> MASWSHPQFEKGAMKHREIRYTDGHTQFVGELHWDEQQGGKCPGVVVFPEAFGLNDHARERARRLAGLGYAALAADLHGDGRLIDDMEQLRPRMEGLFGDRAAWRALARAALDTLVAQPEVDADRLAAIGFCFGGTTALELARS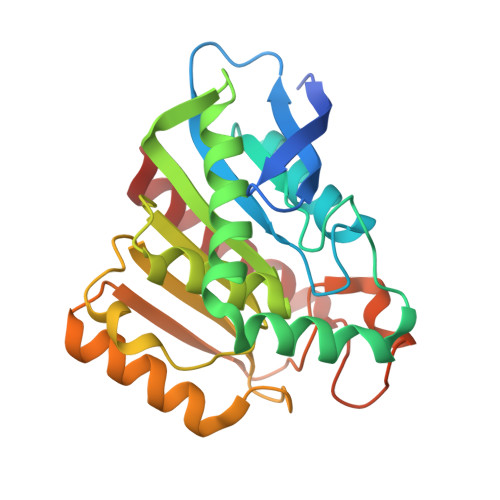GASLGAIVTFHAGLLPELPEDAGRIRGRVLVCHGAEDPLVQKEAIDAVMGEWRRDRVDWQFTFYGNAAHSFTDPAADAHGMAGLAYEPLTEARSWTAMRNLFDEVFSR>[2x]NGNSLSAAELTCGMIMCLARQIPQATASMKDGKWERKKFMGTELNGKTLGILGLGRIGREVATRMQSFGMKTIGYDPIISPEVSASFGVQQLPLEEIWPLCDFITVHTPLLPSTTGLLND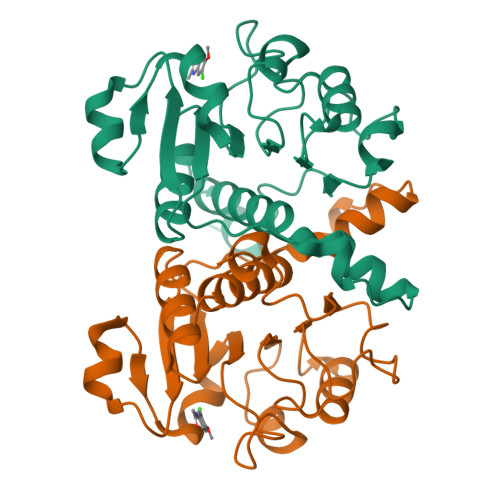NTFAQCKKGVRVVNCARGGIVDEGALLRALQSGQCAGAALDVFTEEPPRDRALVDHENVISCPHLGASTKEAQSR> MDSRLQEIRERQKLRRQLLAQQLGAESADSIGAVLNSKDEQREIAETRETCRASYDTSAPNAKRKYLDEGETDEDKMEEYKDELEM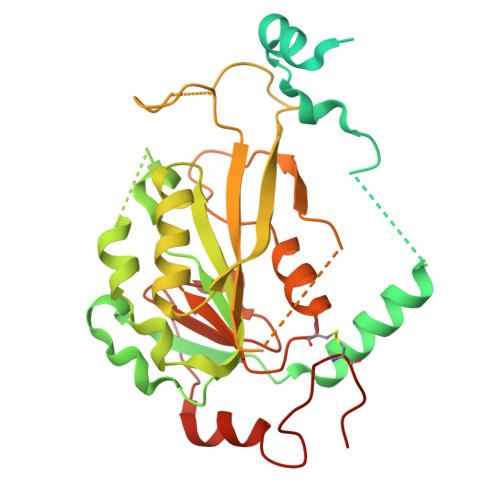QQDEENLPYEEEIYKDSSTFLKGTQSLNPHNDYCQHFVDTGHRPQNFIRDVGLADRFEEYPKLRELIRLKDELIAKSNTPPMYLQADIEAFDIRELTPKFDVILLEPPLEEYYRETGITANEKCWTWDDIMKLEIDEIAAPRSFIFLWCGSGEGLDLGRVCLRKWGYRRCEDICWIKTNKNNPGKTKTLDPKAVFQRTKEHCLMGIKGTVKRSTDGDFIHANVDIDLIITEEPEIGNIEKPVEIFHIIEHFCLGRRRLHLFGRDSTIRPGWLTVGPTLTNSNYNAETYASYFSAPNSYLTGCTEEIERLRPKS> ANIAPRTVFFTIGSSELSPREEMNLSYLAAKMKEFPDTQYTVYGYADSATGTPAFNKELSQKRAQAVVNALVKKYGVDSSRLKVD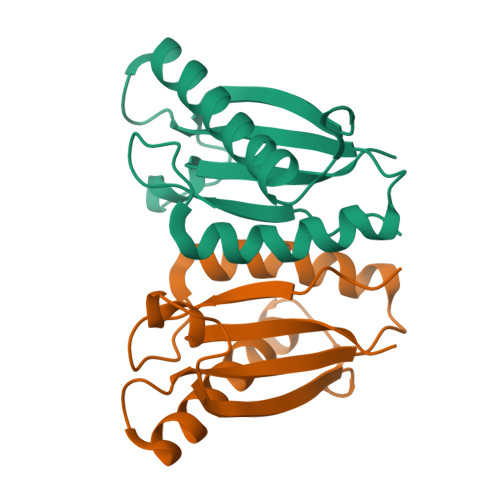AGGGVDKFGKPIYLNRVVLVESVK>[2x]GMAVECIKDKVTRYPERASYSDEDLVAMLDRNFTCTVSFIDGGIPYAIPMMLASEGKTIYLHGSMKSRIYGILKTG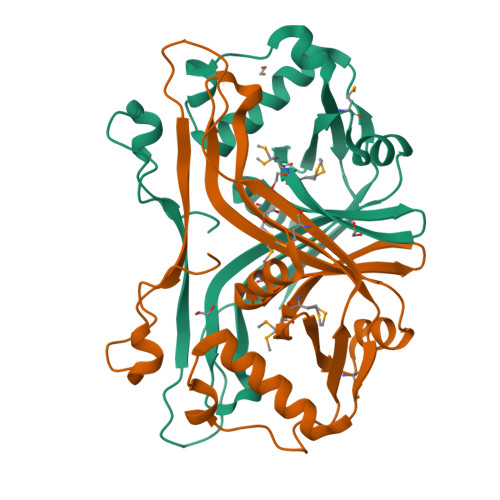QLIAISLLEINGIVLAKEIKNNSINYVSALIFGRPYEIDDTEKKIEVFRLLTEKLVKGRWDNSIKPSYEDLNGVFVFAVKPETFSMKARTGPPHDTSTDDIWSGVLPIQHTISEAGENAPEYVKSLYGKRIFI>PSVRPFKQRKSLAIRQEEVAGIRAKFPNKIPVVVERYPRETFLPPLDK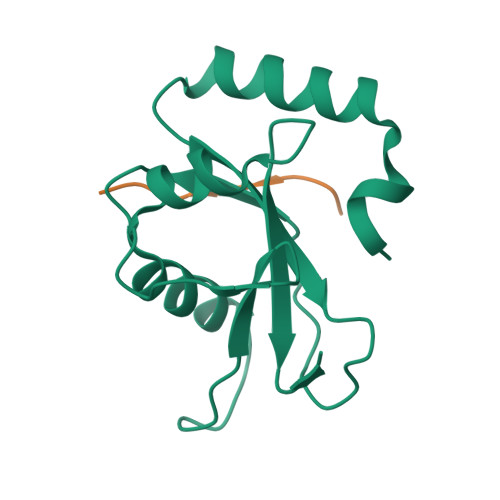TKFLVPQELTMTQFLSIIRSRMVLRATEAFYLLVNNKSLVSMSATMAEIYRDYKDEDGFVYMTYASQETF[8x];>[8x]PQQEDEWVNVQYPD> AGPWADIMQGPSESFVDFANRLIKAVEGSDLPPSARAPVIID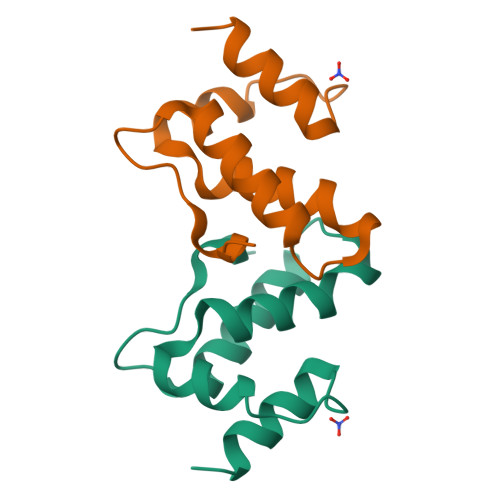CFRQKSQPDIQQLIRTAPSTLTTPGEIIKYVLDRQ> MSNIFLELQDGDKTVYTHTSLIEESKQEQIQAIYDKVPQWTNGGRFLGFWLSMEAVNRVQSVAKLPIYYRAGIVATSTLLGGLVSSLVFWKSGNENQVAKLANGAPVYL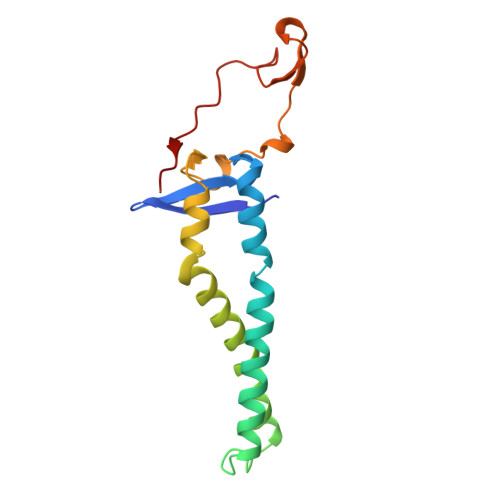KKWEVPELSKLYFFLDDDNNFKPSLNHHAVTQGRQYYKIYQHN> MAGQTTVDSRRQPPEEVDVLVVGAGFSGLYALYRLRELGRSVHVIETAGDVGGVWYWNRYPGARCDIESIEYCYSFSEEVLQEWNWTERYASQPEILRYINFVADKFDLRSGITFHTTVTAAAFDEATNTWTVDTNHGDRIRARYLIMASGQLSVPQLPNFPGLKDFAGNLYHTGNWPHEPVDFSGQRVGVIGTGSSGIQVSPQIAKQAAELFVFQRTPHFAVPARNAPLDPEFLADLKKRYAEFREESRNTPGGTHRYQGPKSALEVSDEELVETLERYWQEGGPDILAAYRDILRDRDANERVAEFIRNKIRNTVRDPEVAERLVP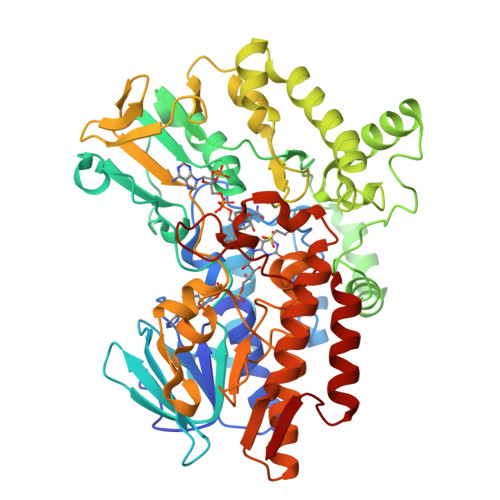KGYPFGTKKLILEIDYYEMFNRDNVHLVDTLSAPIETITPRGVRTSEREYELDSLVLATGFDALTGALFKIDIRGVGNVALKEKWAAGPRTYLGLSTAGFPNLFFIAGPGSPSALSNMLVSIEQHVEWVTDHIAYMFKNGLTRSEAVLEKEDEWVEHVNEIADETLYPMTASWYTGANVPGKPRVFMLYVGGFHRYRQICDEVAAKGYEGFVLT>MQVAPTSSPAGPVSAIPSVFETLQGYKVPVFFSRYPAGISIAAQEVEDALRKIDEEASEEGTRERRRALIRHTNPYGDPFTICHCSAFPDRLALLSCLVEVMWIHDDVTEEMDHISACREHDELAKVLQLDIDPSKFESGNVRQKSLAVVLRKAIDIDPKQAPAMIEMLRHYLATFDNIGGDFTRMEEYMPYRIANCGYWMSSYFIRWGMDMTLSEEEYASIEQFDIAMGNVLGLTNDYFSWNIEKDQETDRMRNGVVVLMKEHHTTADAAKMMLLGVIVEQESLAAKLKEERLKKPASKEILQYFEAIELYVGGSC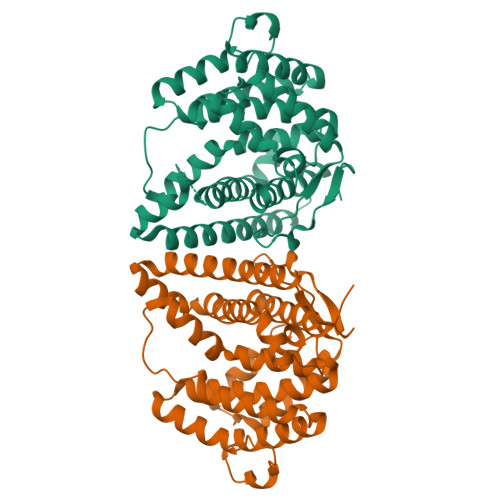YWHSTAPRYQVFE[2x]>[2x]LEFPGAEGQWTRFPKWNACCESEMSFQLKTRSARGLVLYFDDEGFCDFLELILTRGGRLQLSFSIFCAEPATLLTDTPVNDGAWHNVRIRRQFRNTTLFIDQVEAKWVEVKSKRRDMTVFSGLFVGGLPPELRAAALKLTLASVREREPFKGWIRDVRVQSSLALPVDSGEVKLDDEPPNSGGGSPCEAGEEGEGGVCLNGGVCSVVDDQAVCDCSRTGFRGKDCSQGKEEYIATFKGSEYFCYDLSQNPIQSSSDEITLSFKTLQRNGLMLHTGKSADYVNLALKNGAVSLVINLGSGAFEALVEPVNGKFNDNAWHDVKVTRNLRQVTISVDGILTTTGYTQEDYTMLGSDDFFYVGGSPSTADLPGSPVSNNFMGCLKEVVYKNNDVRLELSRLAKQGDPKMKIHGVVAFKCENVATLDPITFETPESFISLPKWNAKKTGSISFDFRTTEPNGLILFSHGKPRHQKDAKHPQMIKVDFFAIEMLDGHLYLLLDMGSGTIKIKALQKKVNDGEWYHVDFQRDGRSGTISVNTLRTPYTAPGESEILDLDDELYLGGLPENKAGLVFPTEVWTALLNYGYVGCIRDLFIDGQSKDIRQMAEVQSTAGVKPSCSRETAKPCLSNPCKNNGMCRDGWNRYVCDCSGTGYLGRSCEREATVLSYDGSMFMKIQLPVVMHTEAEDVSLRFRSQRAYGILMATTSRDSADTLRLELDAGRVKLTVNLGKGPETLFAGYNLNDNEWHTVRVVRRGKSLKLTVDDQQAMTGQMAGDHTRLEFHNIETGIITERRYLSSVPSNFIGHLQSLTFNGMAYIDLCKNGDIDYCELNARFGFRNIIADPVTFKTKSSYVALATLQAYTSMHLFFQ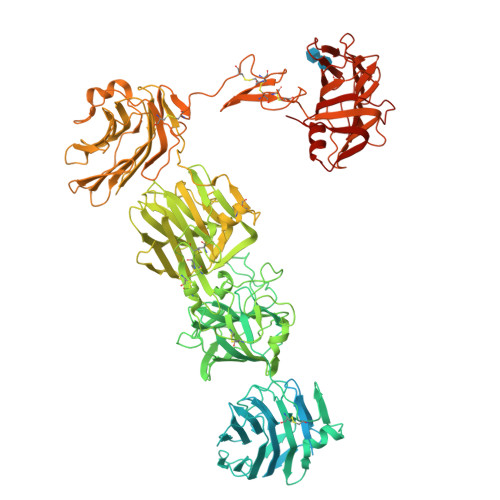FKTTSLDGLILYNSGDGNDFIVVELVKGYLHYVFDLGNGANLIKGSSNKPLNDNQWHNVMISRDTSNLHTVKIDTKITTQITAGARNLDLKSDLYIGGVAKETYKSLPKLVHAKEGFQGCLASVDLNGRLPDLISDALFCNGQIERGCEGPSTTCQEDSCSNQGVCLQQWDGFSCDCSMTSFSGPLCNDPGTTYIFSKGGGQITYKWPPNDRPSTRADRLAIGFSTVQKEAVLVRVDSSSGLGDYLELHIHQGKIGVKFNVGTDDIAIEESNAIINDGKYHVVRFTRSGGNATLQVDSWPVIERYPAGRQLTIFNSQATIIIGGKEQGQPFQGQLSGLYYNGLKVLNMAAENDANIAIVGNVRLVGEVPSASTSHHHHHH>[16x]STEDEGEDPWYQKACKCDCQGGPNALWSAGATSLDCIPECPYHKPLGFESGEVTPDQITCSNPEQYVGWYSSWTANKARLNSQGFGCAWLSKFQDSSQWLQIDLKE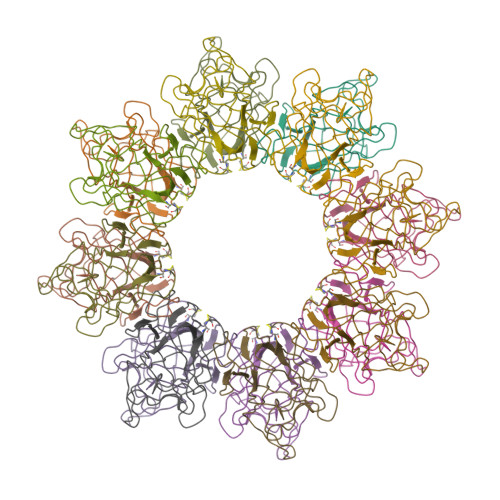IKVISGILTQGHCDIDEWMTKYSVQYRTDERLNWIYYKDQTGNNRVFYGNSDRTSTVQNLLRPPIISRFIRLIPLGWHVRIAIRMELLECVSKCA>[4x]STPSIVIASAARTAVGSFNGAFANTPAHELGATVISAVLERAGVAAGEVNEVILGQVLPAGEGQNPARQAAMKAGVPQEATAWGMNQLCGSGLRAVALG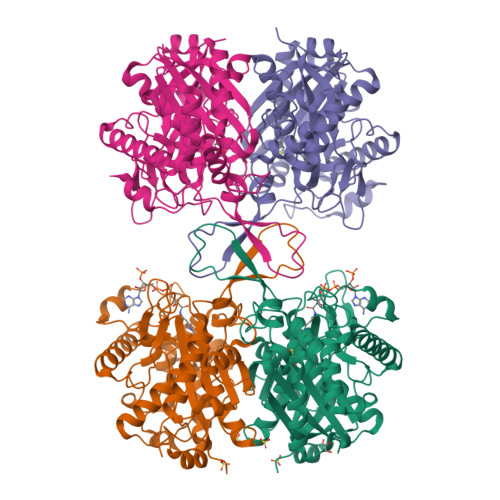MQQIATGDASIIVAGGMESMSMAPHCAHLRGGVKMGDFKMIDTMIKDGLTDAFYGYHMGTTAENVAKQWQLSRDEQDAFAVASQNKAEAAQKDGRFKDEIVPFIVKGRKGDITVDADEYIRHGATLDSMAKLRPAFDKEGTVTAGNASGLNDGAAAALLMSEAEASRRGIQPLGRIVSWATVGVDPKVMGTGPIPASRKALERAGWKIGDLDLVEANEAFAAQACAVNKDLGWDPSIVNVNGGAIAIGHPIGASGARILNTLLFEMKRRGARKGLATLCIGGGMGVAMCIESL> MANVIKTVLTYQLDGSNRDFNIPFEYLARKFVVVTLIGVDRKVLTINTDYRFATRTTISLTKAWGPADGYTTIELRRVTSTTDRLVDFTDGSILRAYDLNVAQIQTMHVAEEARDLTTDTIGVNNDGHLDARGRRIVNLANAVDDRDAVPFGQLKTMNQNSWQARNEALQFRNEAETFRNQAEGFKNESSTNATNTKQWRDETKGFRDEAKRFKNTAGQYATSAGNSA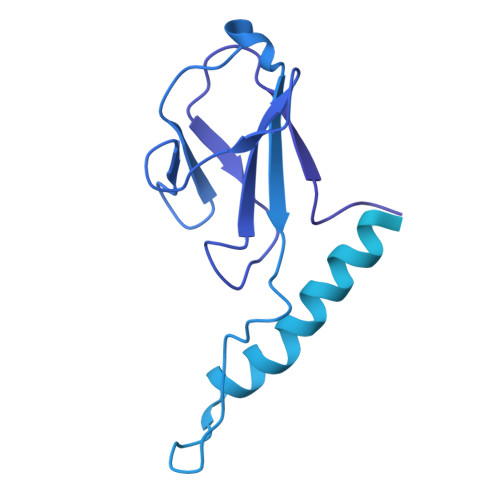SAAHQSEVNAENSATASANSAHLAEQQADRAEREADKLENYNGLAGAIDKVDGTNVYWKGNIHANGRLYMTTNGFDCGQYQQFFGGVTNRYSVMEWGDENGWLMYVQRREWTTAIGGNIQLVVNGQIITQGGAMTGQLKLQNGHVLQLESASDKAHYILSKDGNRNNWYIGRGSDNNNDCTFHSYVHGTTLTLKQDYAVVNKHFHVGQAVVATDGNIQGTKWGGKWLDAYLRDSFVAKSKAWTQVWSGSAGGGVSVTVSQDLRFRNIWIKCANNSWNFFRTGPDGIYFIASDGGWLRFQIHSNGLGFKNIADSRSVPNAIMVENE> MDGVHDLAGVQGFGKVPHTVNADIGPTFHAEWEHLPYSLMFAGVAELGAFSVDEVRYVVERMEPRHYMMTPYYERYVIGVATLMVEKGILTQDELESLAGGPFPLSRPSESEGRPAPVE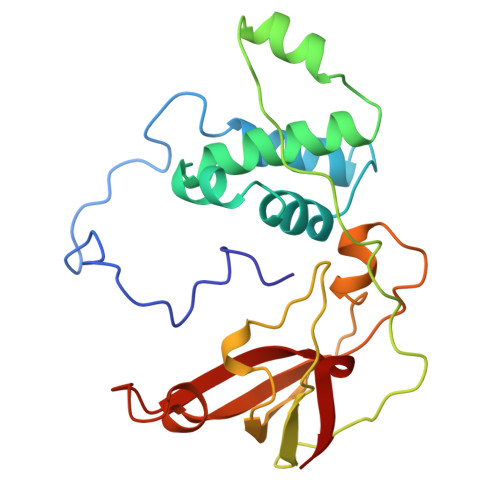TTTFEVGQRVRVRDEYVPGHIRMPAYCRGRVGTISHRTTEKWPFPDAIGHGRNDAGEEPTYHVKFAAEELFGSDTDGGSVVVDLFEGYLEPAA> GSGGEQAQDWDALPPKRPRLGAGNKIGGRRLIVVLEGASLETVKVGKTYELLNCDKHKSILLKNGRDPGEARPDITHQSLLMLMDSPLNRAGLLQVYIHTQKNVLIEVNPQTRIPRTFDRFCGLMVQLLHKLSVRAADGPQKLLKVIK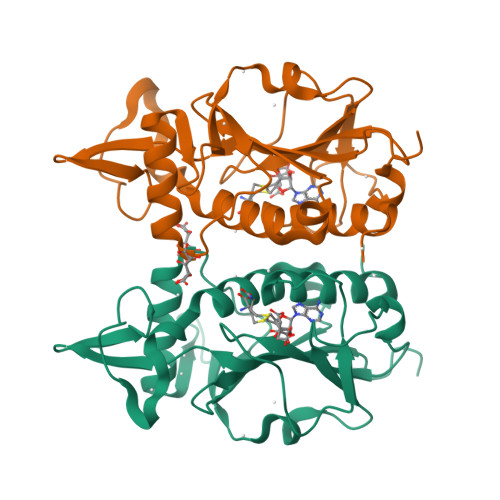NPVSDHFPVGCMKVGTSFSIPVVSDVRELVPSSDPIVFVVGAFAHGKVSVEYTEKMVSISNYPLSAALTCAKLTTAFEEVWGVI> PPQPRKKRPEDFKFGKILGEGSFSTVVLARELATSREYAIKILEKRHIIKENKVPYVTRERDVMSRLDHPFFVKLYFTFQDDEKLYFGLSYAKNGELLKYIRKIGSFDETCTRFYTAEIVSALEYLHGKGIIHRDLKPENILLNEDMHIQITDFGTAKVLSPESKQARANSFVGTAQYVSPELLTEKSACKSSDLWALGCIIYQLVAGLPPFRAGNEYLIFQKIIKLEYDF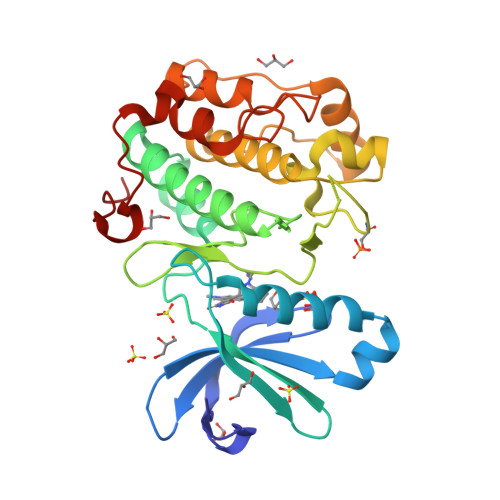PEKFFPKARDLVEKLLVLDATKRLGCEEMEGYGPLKAHPFFESVTWENLHQQTPPKLT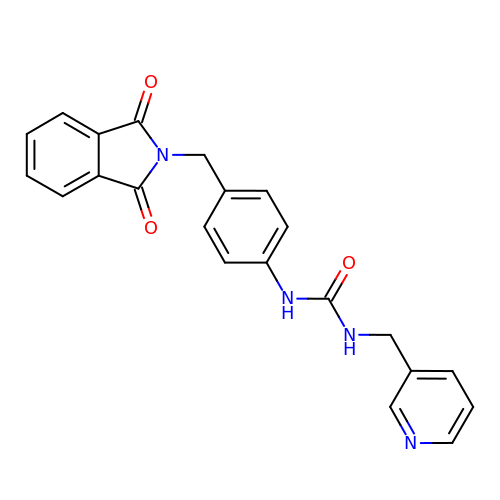N-{4-[(1,3-dioxo-1,3-dihydro-2H-isoindol-2-yl)methyl]phenyl}-N'-[(pyridin-3-yl)methyl]urea | C22 H18 N4 O3 | KKBVILNJYCRNQY-UHFFFAOYSA-N> SYRHFA;> MHHHHHHMQIGWRREGIKYRRNELFLDVLESVNLLMSPQGQVLSAHVSGRVVMKSYLSGMPECKFGMNDKIVIEKQGKGTADETSKSGKQSIAIDDCTFHQCVRLSKFDSERSISFIPPDGEFELMRYRTTKDIILPFRVIPLVREVGRTKLEVKVVIKSNFKPSLLAQKIEVRIPTPLNTSGVQVICMKGKAKYKASENAIVWKIKRMAGMKESQISAEIELLPTNDKKKWARPPISMNFEVPFAPSGLKVRYLKVFEPKLNY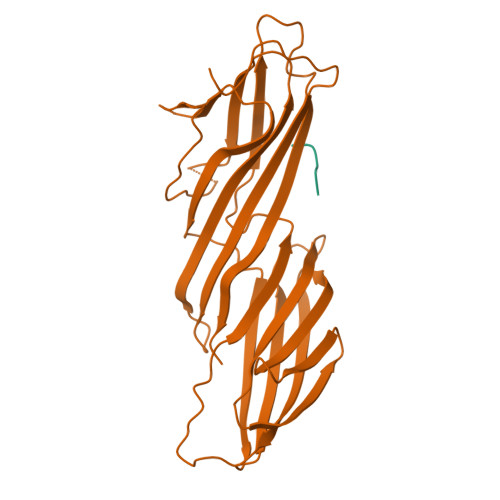SDHDVIKWVRYIGRSGIYETRC> MKDEVALLAAVTLLGVLLQAYFSLQVISARRAFRVSPPLTTGPPEFERVYRAQVNCSEYFPLFLATLWVAGIFFHEGAAALCGLVYLFARLRYFQGYARSAQLRLAPLYASARALWLLVALAALGLLAHFLPAALRAALLG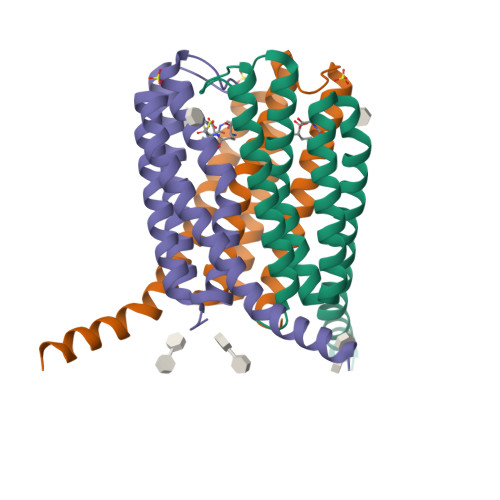RLRTLLPWAHHHHHH>XGEIAQALKEIAKATKEIAWATKEIAQA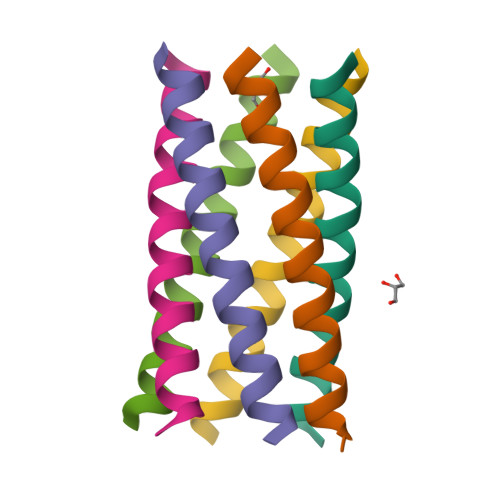LKGX[6x]> YDGT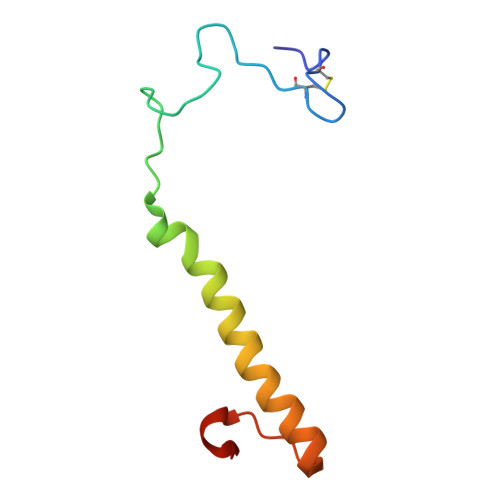KCKAAGNCWEPKPGFPEKIAGSKYDPKHDPKELNKQADSIKQMEERNKKRVENFKKTGKFEYDVAKISAN>LKPPSMYKVILVNDDYTPMEFVIDVLQKFFSYDVERATQLMLAVHYQGKAICGVFTAEVAETKVAMVNK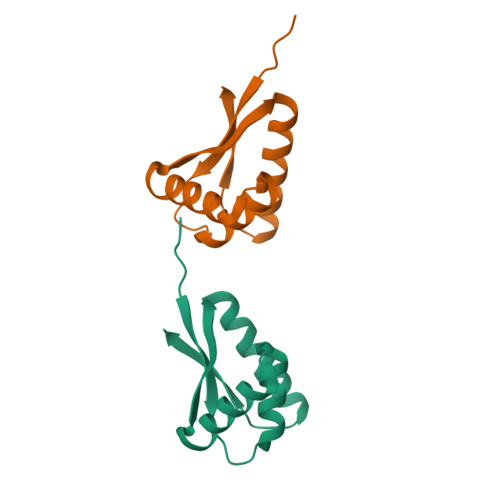YARENEHPLLCTLEKA[8x]>[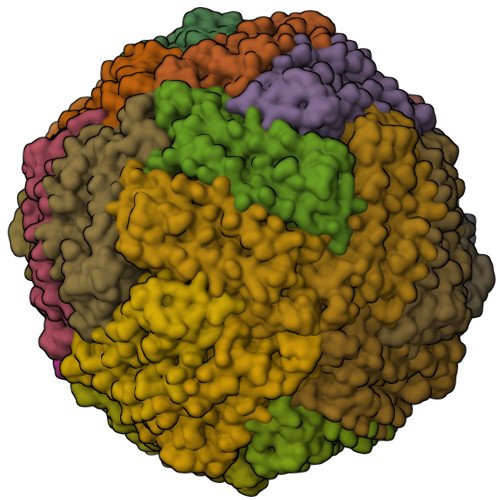24x]SQIRQNYSTEVEAAVNRLVNLYLRASYTYLSLGFYFDRDDVALEGVCHFFRELAEEKREGAERLLKMQNQRGGRALFQDLQKPSQDEWGTTLDAMKAAIVLEKSLNQALLDLHALGSAQADPHLCDFLESHFLDEEVKLIKKMGDHLTNIQRLVGSQAGLGEYLFERLTLK>[4x]MLMTAEQYIESLRKLNTRVYMFGEKIENWVDHPMIRPSINCVRMTYELAQDPQYADLMTTKSNLIGKTINRFANLHQSTDDLRKKVKMQRLLGQKTASCFQRCVGMDAFNAVFSTTYEIDQKYGTNYHKNF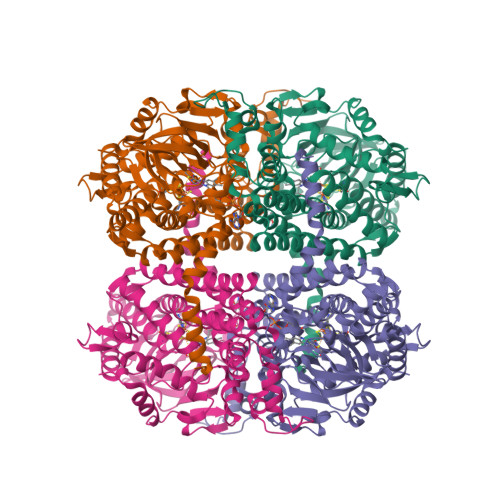TEYLKYIQENDLIVDGAMTDPKGDRGLAPSAQKDPDLFLRIVEKREDGIVVRGAKAHQTGSINSHEHIIMPTIAMTEADKDYAVSFACPSDADGLFMIYGRQSCDTRKMEEGADIDLGNKQFGGQEALVVFDNVFIPNDRIFLCQEYDFAGMMVERFAGYHRQSYGGCKVGVGDVVIGAAALAADYNGAQKASHVKDKLIEMTHLNETLYCCGIACSAEGYPTAAGNYQIDLLLANVCKQNITRFPYEIVRLAEDIAGGLMVTMPSEADFKSETVVGRDGETIGDFCNKFFAAAPTCTTEERMRVLRFLENICLGASAVGYRTESMHGAGSPQAQRIMIARQGNINAKKELAKAIAGIK> MDNSHDSDSVFLYHIPCDNCGSSDGNSLFSDGHTFCYVCEKWTAGNEDTKERASKRKPSGGKPMTYNVWNFGESNGRYSALTARGISKETCQKAGYWIAKVDGVMYQVADYRDQNGNIVSQKVRDKDKNFKTTGSHKSDALFGKHLWNGGKKIVVTEGEIDMLTVMELQDCKYPVVSLGHGASAAKKTCAANYEYFDQFEQIILMFDMDEAGRKAVEEAAQVLPAG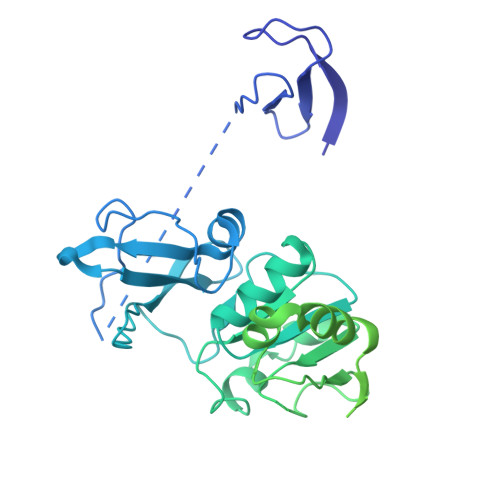KVRVAVLPCKDANECHLNGHDREIMEQVWNAGPWIPDGVVSALSLRERIREHLSSEESVGLLFSGCTGINDKTLGARGGEVIMVTSGSGMGKSTFVRQQALQWGTAMGKKVGLAMLQESVEETAEDLIGLHNRVRLRQSDSLKREIIENGKFDQWFDELFGNDTFHLYDSFAEAETDRLLAKLAYMRSGLGCDVIILDHISIVVSASGESDERKMIDNLMTKLKGFAKSTGVVLVVICHLKNPDKGKAHEEGRPVSITDLRGSGALRQLSDTIIALERNQQGDMPNLVLVRILKCRFTGDTGIAGYMEYNKETGWLEPSSYSGEEESHSESTDWSNDTDF2-{5-[AMINO(IMINIO)METHYL]-6-CHLORO-1H-BENZIMIDAZOL-2-YL}-6-ISOBUTOXYBENZENOLATE 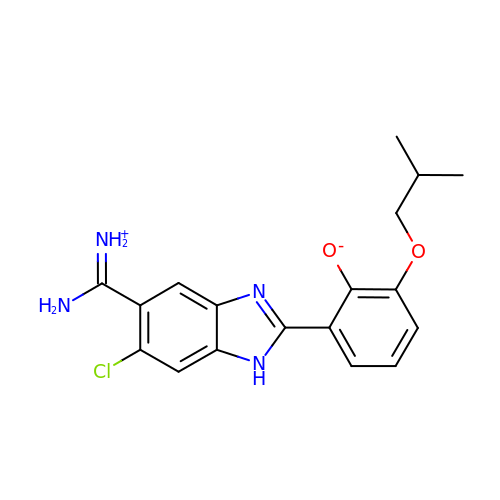| C18 H19 Cl N4 O2 | RTSLVPMQUZXPBZ-UHFFFAOYSA-N>MYFQIRGIILWPRNKNFKPHTIRFELGKVNVISGASRTGKSAVIPIIDYCLGANTCSIPVKTIRKYCEWFGIVVATEQGEKLLARKEPGNQRSTTDMFVLEAENITSIPIRLEKNTNVIAVKRMLDDLANLSNLDFSGGDENSGFDGRPAFRDLAAFTFQPQNVVANPDVLFFKTNTYEHREKLRKIFPYVLGAITSELMAKQFELNRIRLFLRRKERELKDAQDVSAQWLADLKSKYSEAQELGLVPKPQEQLSRKQMISQLEEVISRTDLTLKVTVSTISDALSELNTLESEERLVSRELTTMRHRLEEMNRLRVGMHQYENALLMQRDRLKISGWLLSNTNDESDCPMCGSHTDSAKQKLQALVQRLSDVEAAVGADAHKEVPAAFDRELQRVTTEVANATERLRAIQSRKRTLTSRSKEAREQQFSTRRAERFIG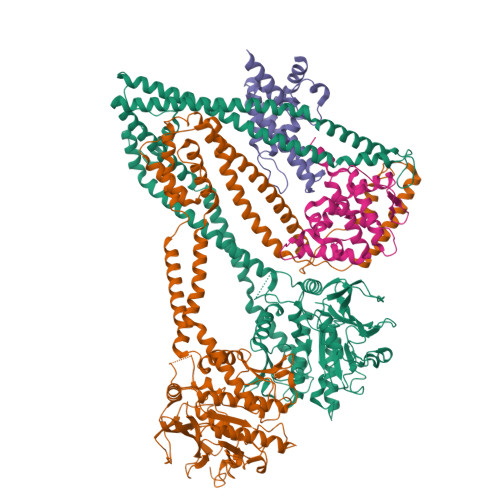NVESALELHRKLGSDSELVEEVRKLKEMVQTLEKELREKDVELRKNQALRVINAQAGNILQGLDVEDPSAPISLEINDLTIKVLGDERDDYLSEIGSGSNWLSYHLAILLSLHQFYLSQKNNPVPSFLILDQPSQVYFPKTTQLPNIANEDEPKLRDEDVEAVRRAFKAMGNVVIKEKGKLQLIVLDHAPREVWGEIDGVVGLPEWRDGIKLVPMEWLTGV[2x];> MAISKTNGQSKPKRKTEVPGQALGYSLQFTLLTHLLLQAPEGSLCSLEVLDDVAQENNSGDIKFIQSKSALTANPAADRAKSLWKTLSNWIDLATSPDFEVEKAIFELYVSRPVEGSIVKKFNEAKTPEDAQEAITHARTELWGDSPHFTLKDGISKEISKYVEKVFTADQNLLQRLICNFQLTLGSGSPQADLEACVRSHPVSPSKVSDITNYLCGKVKRHIDMLLEAEKPAVIARDDFYTWYKAYVQKIDRQMVLSSRAQAPVKEKAQEYLPDKFVQQLEIIGLPYEEILGAISDYLMASFDRTDWAARGEVDETSFDDLDTALQRTWKNKQRICGLTHSEKSEQDQGKLLYFECMQFNIPLQAMSPPSHFIPGCYHILADSLAVGWHPNYTTQLKNKKVA;> MLAREAQNIQNPALGAALVWRFCCGYVKTNRVSAPPPLPFLFLVLPIILHQETSEFVKRTYKSSGLRAFAAKFGDSSVSKQDLLFQIHERSIRWRQLSLRSIELAVASDLLKLQDGSDVIPLSKTKARGLSDEVKTLMDLAEKLGSWFGELSIHEVVTTLKVKL>GAQNFSDYFTNKTLRIDYLFTGNADKQSICLDELSELPVWAGRRHHLSELPLEGNGQIVMRDVASGKVIYTTSFSSLFQEWLETDEAKEVTKGFENTYLLPYPIKPAEVEITLRNNKREVSANLKHVVKPDDILIHKKGLTHITPHKYLLKSGNEEQCIDVAILAEGYTTSEMETFYKDAAIACEALFSHEPFQSMKNRFNIVAVASPSADSGVSAPKQGAWKHTAFGSHFDTFYSDRYLTTSRVKAINDALAGIPYEHIIILANTEQYGGGGIYNAFTLTTAHHPNFRPVVVHEFGHSFGGLADEYFYDEDVMNGLYPLNIEPWEQNITTRINFASKWEDMLTKTTPVPTPVADKAKYPIGVYEGGGYSAKGIYRPAFDCRMRTNEYPT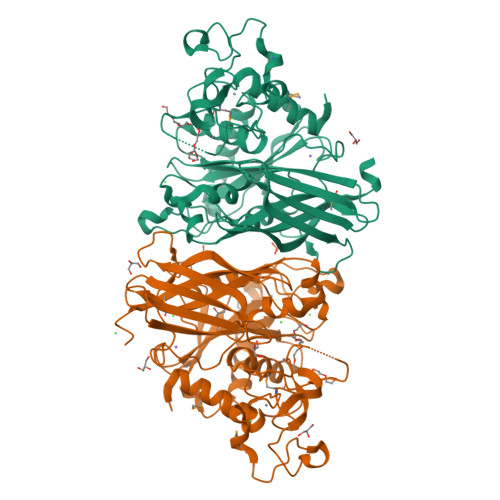FCPVCQRAIQRIIEFYTGK[6x]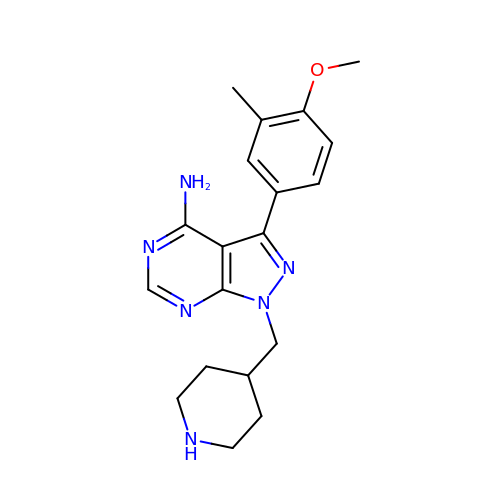3-(4-methoxy-3-methylphenyl)-1-(piperidin-4-ylmethyl)-1H-pyrazolo[3,4-d]pyrimidin-4-amine | C19 H24 N6 O | MQULVMDBNSSIMR-UHFFFAOYSA-N3-{[(1R,2S)-2-aminocyclohexyl]amino}-5-(1H-indol-7-ylamino)-1,2,4-triazine-6-carboxamide 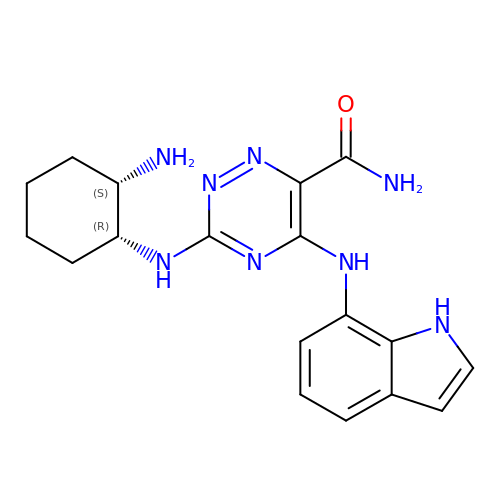| C18 H22 N8 O | FPQNRXITKTZFMF-NWDGAFQWSA-N>[3x]MKNWKTSAESILTTGPVVPVIVVKKLEHAVPMAKALVAGGVRVLEVTLRTECAVDAIR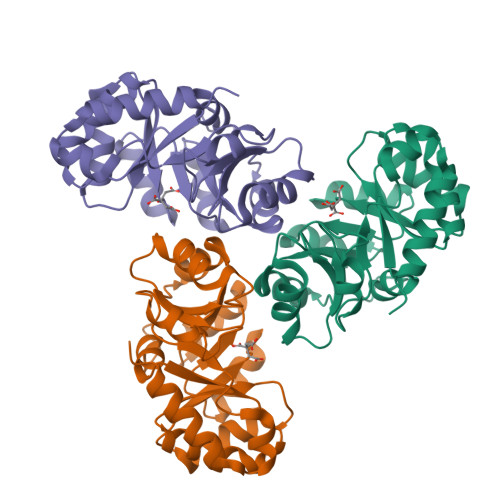AIAKEVPEAIVGAGTVLNPQQLAEVTEAGAQFAISPGLTEPLLKAATEGTIPLIPGISTVSELMLGMDYGLKEFQFFPAEANGGVKALQAIAGPFSQVRFCPKGGISPANYRDYLALKSVLCIGGSWLVPADALEAGDYDRITKLAREAVEGAKL>MADIGSTYNGPLSSHWF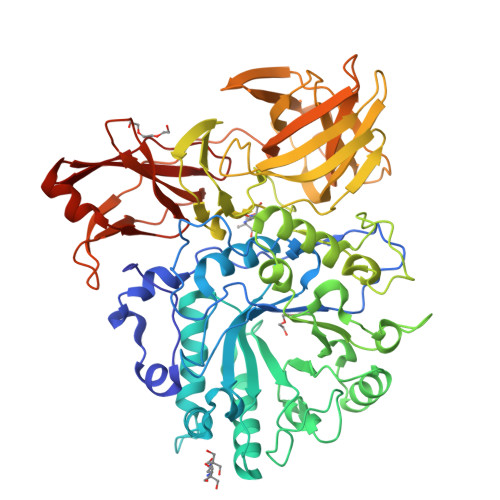PEELAQWEPDSDPDAPFNRSHVPLEPGRVADRVNANADTDAHLVSLSALNRHTSGVPSQGAPVFYENTFSYWHYTDLMVYWAGSAGEGIIVPPSADVIDASHRNGVPILGNVFFPPTVYGGQLEWLEQMLEQEEDGSFPLADKLLEVADYYGFDGWFINQQTEGADEGTAEAMQAFLVYLQEQKPEGMHIMWYDSMIDTGAIAWQNHLTDRNKMYLQNGSTRVADSMFLNFWWRDQRQSNELAQALGRSPYDLYAGVDVEARGTSTPVQWEGLFPEGEKAHTSLGLYRPDWAFQSSETMEAFYEKELQFWVGSTGNPAETDGQSNWPGMAHWFPAKSTATSVPFVTHFNTGSGAQFSAEGKTVSEQEWNNRSLQDVLPTWRWIQHGGDLEATFSWEEAFEGGSSLQWHGSLAEGEHAQIELYQTELPISEGTSLTWTFKSEHGNDLNVGFRLDGEEDFRYVEGEQRESINGWTQWTLPLDAFAGQTITGLAFAAEGNETGLAEFYIGQLAVGADSEKPAAPNVNVRQYDPDPSGIQLVWEKQSNVHHYRVYKETKHGKELIGTSAGDRIYLEGLVEESKQNDVRLHIEALSETFVPSDARMIDIKSGSF[2x]>[3x]GPGSMSAARELLVERDGPVVILTMNRPHRRNALSTNMVSQFAAAWDEIDHDDGIRAAILTGAGSAYCVGGDLSDGWMVRDGSAPPLDPATIGKGLLLSHTLTKPLIAAVNGACLGGGCEMLQQTDIRVSDEHATFGLPEVQRGLVPGAGSMVRLKRQIPYTKAMEMILTGEPLTAFEAYHFGLVGHVVPAGTALDKARSLADRIVRNGPLAVRNAKEAIVRSGWLAEEDARAIEARLTRPVITS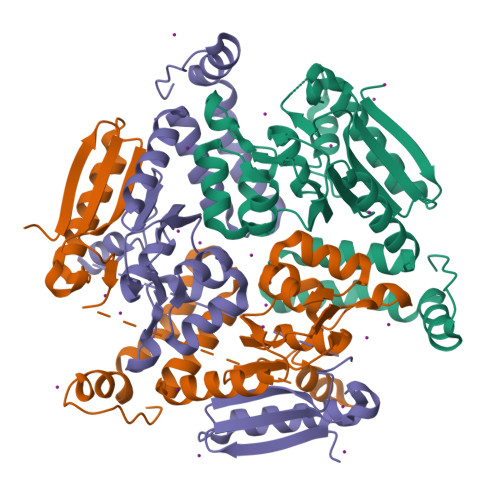ADAREGLAAFKEKREARFTGR>[3x]G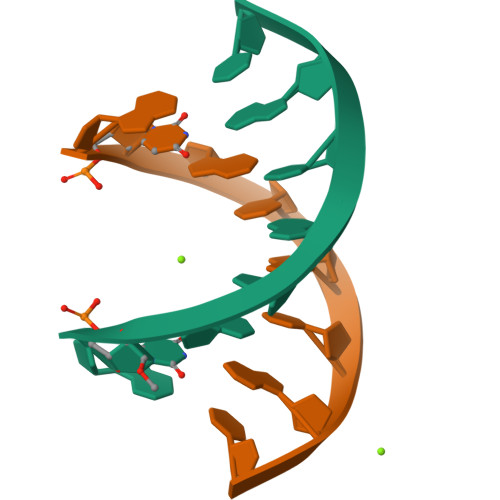UGTXCAC N-[(1S,2R)-2-aminocyclohexyl]-4-[6-(1-methyl-1H-pyrazol-4-yl)pyrazolo[1,5-a]pyrimidin-3-yl]thiophene-2-carboxamide | C21 H23 N7 O S | 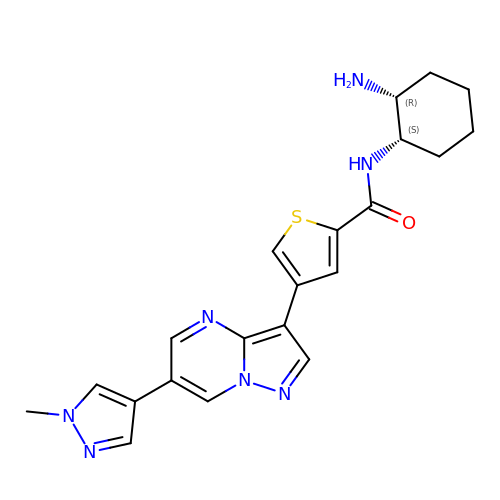LYADGAGFYYXXIO-MSOLQXFVSA-N N-[(2R)-tetrahydrofuran-2-ylmethyl]cyclohexanecarboxamide | 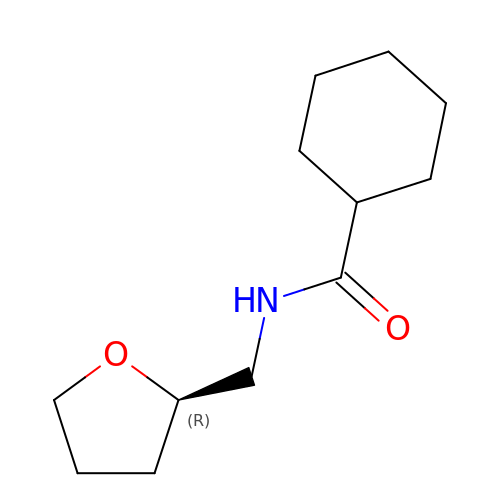C12 H21 N O2 | VZZZJFZRZIRFPP-LLVKDONJSA-N>TGDTTDDDKVDTTIKPIEYPKPDGCNRTGDHFTMEPGANFYTVPNLGPASSNSDECYTNPSFSIGSSIYMFSQEIRKTDCTAGEILSIQIVLGRIVDKGQQGPQASPLLVWAVPNPKIINSCAVAAGDEMGWVLCSVTLTAASGEPIPHMFDGFWLYKLEPDTEVVSYRITGYAYLLDKQYDSVFIGKGGGIQKGNDLYFQMYGLSRNRQSFKALCEHGSCLGTGGGGYQVLCDRAVMSFGSEESLITNAYLKVNDLASGKPVIIGQTFPPSDSYKGSNGRMYTIGDKYGLYLAPSSWNRYLRFGITPDISVRSTTWLKSQDPIMKILSTCTNTDRDMCPEICNTRGYQDIFPLSEDSEYYTYIGITPNNGGTKNFVAVRDSDGHIASIDILQNYYSITSATISCFMY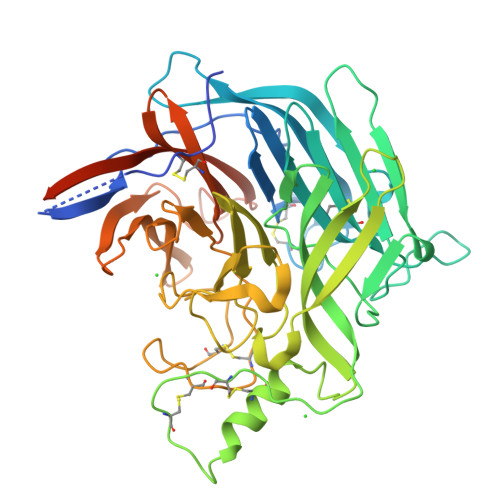KDEIWCIAITEGKKQKDNPQRIYAHSYKIRQMCYNMKSATVTVGNAKNITIRRYGTKHHHHHH[2x]> GRAMGACSHGPVDVVFLLHATRDNAHNAEAVRRVLERLVSALGPLGPQAAQVGLLTYS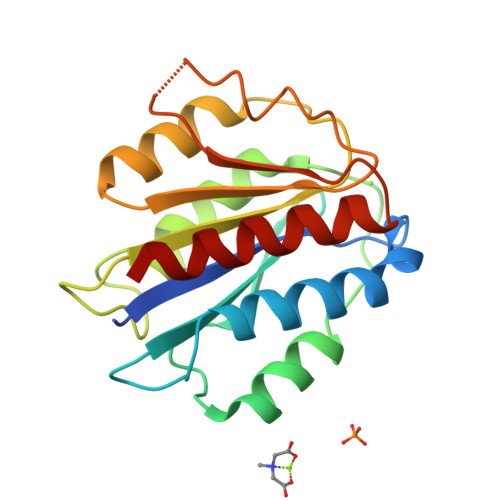HRPSPLFPLNSSHDLGIILRKIRDIPYVDPSGNNLGTAVTTAHRYLLASNAPGRRQQVPGVMVLLVDEPLRGDILSPIREAQTSGLKVMALSLVGADPEQLRRLAPGTDPIQNFFAVDNGPGLDRAVSDLAVALCQAA> KPQVTILATGGTIAGSAGAVTVDKLLAAVPAINDLATIKGEQISSIGSQEMTGKVWLKLAKRVNELLAQKETEAVIITHGTDTMEETAFFLNLTVKSQKPVVLVGAMRPGSSMSADGPMNLYNAVNVAINKASTNKGVVIVMNDEIHAAREATKLNTTAVNAFASPNTGKIGTVYYGKVEYFTQSVRPHTLASEFDISKIEELPRVDILYAHPDDTDVLVNAALQAGAKGIIHAGMGNGNPFPLTQNALEKAAKSGVVVARSSRVGSGSTTQEAEVDDKKLGFVATESLNPQKARVLLMLALTKTSDREAIQKIFSTY;> KPQVTILATGGTIAGVTVDKLLAAVPAINDLATIKGEQISSIGSQEMTGKVWLKLAKRVNELLAQKETEAVIITHGTDTMEETAFFLNLTVKSQKPVVLVGAMRPGSSMSADGPMNLYNAVNVAINKASTNKGVVIVMNDEIHAAREATKLNTTAVNAFASPNTGKIGTVYYGKVEYFTQSVRPHTLASEFDISKIEELPRVDILYAHPDDTDVLVNAALQAGAKGIIHAGMGNGNPFPLTQNALEKAAKSGVVVARSSRVGSGSTTQEAEVDDKKLGFVATESLNPQKARVLLMLALTKTSDREAIQKIFSTY;> KPQVTILATGGTIAGAVTVDKLLAAVPAINDLATIKGEQISSIGSQEMTGKVWLKLAKRVNELLAQKETEAVII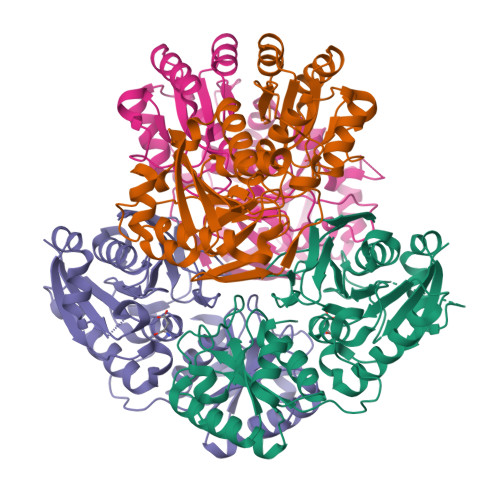THGTDTMEETAFFLNLTVKSQKPVVLVGAMRPGSSMSADGPMNLYNAVNVAINKASTNKGVVIVMNDEIHAAREATKLNTTAVNAFASPNTGKIGTVYYGKVEYFTQSVRPHTLASEFDISKIEELPRVDILYAHPDDTDVLVNAALQAGAKGIIHAGMGNGNPFPLTQNALEKAAKSGVVVARSSRVGSGSTTQEAEVDDKKLGFVATESLNPQKARVLLMLALTKTSDREAIQKIFSTY;> KPQVTILATGGTIAGSGAVTVDKLLAAVPAINDLATIKGEQISSIGSQEMTGKVWLKLAKRVNELLAQKETEAVIITHGTDTMEETAFFLNLTVKSQKPVVLVGAMRPGSSMSADGPMNLYNAVNVAINKASTNKGVVIVMNDEIHAAREATKLNTTAVNAFASPNTGKIGTVYYGKVEYFTQSVRPHTLASEFDISKIEELPRVDILYAHPDDTDVLVNAALQAGAKGIIHAGMGNGNPFPLTQNALEKAAKSGVVVARSSRVGSGSTTQEAEVDDKKLGFVATESLNPQKARVLLMLALTKTSDREAIQKIFSTY>[4x]MVPRRTTNDGFHLLKAGGSCFALI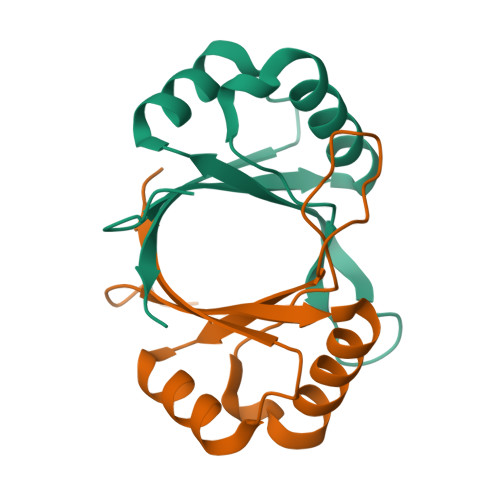SGTANQVKCYRFRVKKNHRHRYENCTTTWFTVADNGAERQGQAQILITFGSPSQRQDFLKHVPLPPGMNISGFTASLDF[(2~{R},3~{S},4~{R},5~{S})-3,4-bis(oxidanyl)-5-[2-(5-phenyl-1,2,3,4-tetrazol-2-yl)ethyl]oxolan-2-yl]methyl 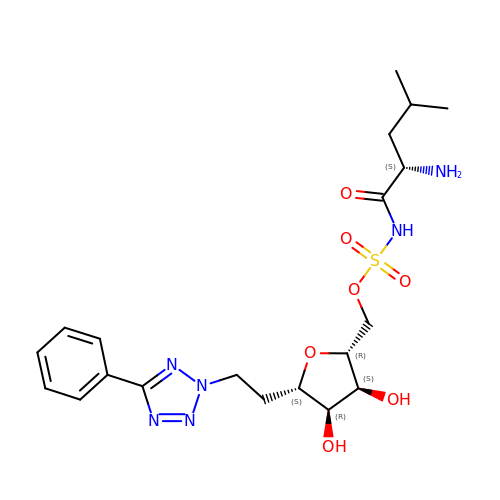~{N}-[(2~{S})-2-azanyl-4-methyl-pentanoyl]sulfamate | C20 H30 N6 O7 S | AWUZSNXCDBPNMM-IECFSIQFSA-N>SMSGISPKKSKYMTPMQQKLNEVYEAVKNYTDKRGRRLSAIFLRLPSRSELPDYYLTIKKPM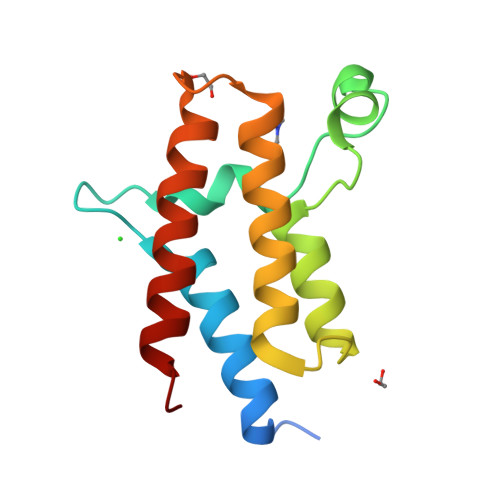DMEKIRSHMMANKYQDIDSMVEDFVMMFNNACTYNEPESLIYKDALVLHKVLLETRRDLEGD[2x]>[2x]GSHMQVTPRRNVLQKRPVIV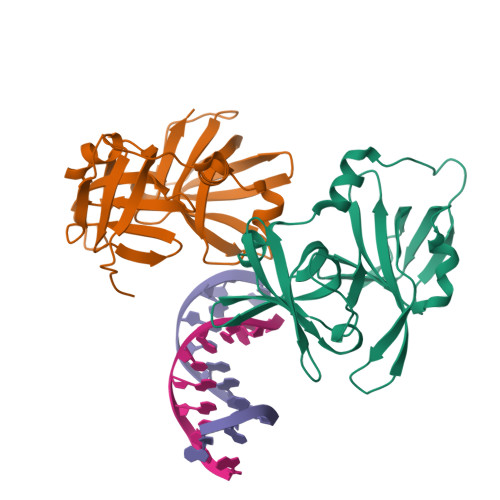KVLSTTKPFEYETPEMEKKIMFHATVATQTQFFHVKVLNTSLKEKFNGKKIIIISDYLEYDSLLEVNEESTVSEAGPNQTFEVPNKIINRAKETLKIDILHKQASGNIVYGVFMLHKKTVNQKTTIYEIQDDRGKMDVVGTGQCHNIPCEEGDKLQLFCFRLRKKNQMSKLISEMHSFIQIKKKTN>GIDPFTMKYVGSIDQGTTSTRFIIFDERQRPVSVHQVPHTQHTPHPGWLEHDPMEIFRSACKCMSVAIAKLRQKDASFRKIEAIGITNQRETTVAWDRVTKEPLCYAPVWNDLRTYDITKKVTAELGGGDSMFASKITGLPVST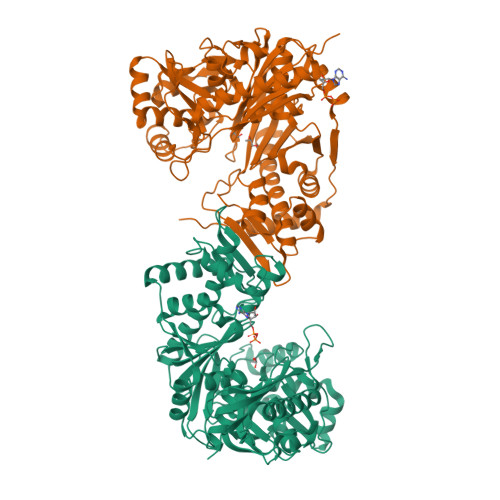YFAAFKMRWMLENVPAVADACRRGTLCFGTIDTWLMYKLSGGKAFVTDVTNASRTFLMDLRTRKWSPELCEKLKIPMETLPEIRSNSELFGYVETDECGVAAALNERTPIMGSIGDQQSALFGNMCFEKGEAKNTYGTGCFLLMNVGEEARFSKHGLLSTVGFQVGRDGPCYYALEGAIACAGATVEWMRRNMNLFSHITECEKLARSVPGTQGIVFVPAFSGLLAPYWDPSARGTIVGMTLKTTRAHVIRAALQAIALQLNDVVGSMKRDAGLNLSSLRVDGGLSKNGLLMEIQASLLGVDILVPSMHETTALGAALCAGLAAGVWTSLEEVKAVSRRENSWKTVSPSGSAMEREAMIAEWREALKRTKWAKL[2x]>MTPESVMMMGTEAMKVALALAAPLLLVALITGLIISILQAATQINEMTLSFIPKIVAVFIAIIVAGPWMLNLLLDYVRTLFSNLPYIIG[4x];> MIQVTSEQWLYWLHLYFWPLLRVLALISTAPILSERAIPKRVKLGLGIMITLVIAPSLPANDTPLFSIAALWLAMQQILIGIALGFTMQFAFAAVRTAGEFIGLQMGLSFATFVDPGSHLNMPVLARIMDMLAMLLFLTFNGHLWLISLLVDTFHTLPIGSNPVNSNAFMALARAGGLIFLNGLMLALPVITLLLTLNLALGLLNRMAPQLSIFVIGFPLTLTVGIMLMAALMPLIAPFCEHLFSEIFNLLADIVSEMPINNNP;>[5x]MRRLLFLSLAGLWLFSPAAAAQLPGLISQPLAGGGQSWSLSVQTLVFITSLTFLPAILLMMTSFTRIIIVFGLLRNALGTPSAPPNQVLLGLALFLTFFIMSPVIDKIYVDAYQPFSEQKISMQEALDKGAQPLRAFMLRQTREADLALFARLANSGPLQGPEAVPMRILLPAYVTSELKTAFQIGFTIFIPFLIIDLVIASVLMALGMMMVPPATIALPFKLMLFVLVDGWQLLMGSLAQSFYS;>MAAIQGIEGVISQLQATAMAARGQDTHSQSTVSFAGQLHAALDRISDRQAAARVQAEKFTLGEPGIALNDVMADMQKASVSMQMGIQVRNKLVAAYQEVMSMQV[6x];>[5x]MLDRLDAALRFQQEALNLRAQRQEILAANIANADTPGYQARDIDFASELKKVMVRGREETGGVALTLTSSHHIPAQAVSSPAVDLLYRVPDQPSLDGNTVDMDRERTQFADNSLKYQMGLTVLGSQLKGMMNVLQGGN;>MALLNIFDIAGSALAAQSKRLNVAASNLANADSVTGPDGQPYRAKQVVFQVDAAPGQATGGVKVASVIESQAPEKLVYEPGNPLADANGYVKMPNVDVVGEMVNTMSASRSYQANIEVLNTVKSMMLKTLTLGQ[6x];>[11x]MSATASTATQPKPLEWLNRLRANPRIPLIVAGSAAVAIVVAMVLWAKTPDYRTLFSNLSDQDGGAIVAQLTQMNIPYRFANGSGAIEVPADKVHELRLRLAQQGLPKGGAVGFELLDQEKFGISQFSEQVNYQRALEGELARTIETLGPVKSARVHLAMPKPSLFVREQKSPSASVTVTLEPGRALDEGQISAVVHLVSSAVAGLPPGNVTLVDQSGHLLTQSNTSGRDLNDAQLKFANDVESRIQRRIEAILSPIVGNGNVHAQVTAQLDFANKEQTEEHYSPNGDASKATLRSRQLNISEQVGAGYPGGVPGALSNQPAPPNEAPIATPPTNQQNAQNTPQTSTSTNSNSAGPRSTQRNETSNYEVDRTIRHTKMNVGDIERLSVAVVVNYKTLADGKPLPLTADQMKQIEDLTREAMGFSDKRGDTLNVVNSPFSAVDNTGGELPFWQQQSFIDQLLAAGRWLLVLVVAWILWRKAVRPQLTRRVEEAKAAQEQAQVRQETEEAVEVRLSKDEQLQQRRANQRLGAEVMSQRIREMSDNDPRVVALVIRQWMSNDHE;>MDHAIYTAMGAASQTLNQQAVTASNLANASTPGFRAQLNALRAVPVDGLSLATRTLVTASTPGADMTPGQLDYTSRPLDVALQQDGWLVVQAADGAEGYTRNGNIQVGPTGQLTIQGHPVIGEGGPITVPEGSEITIAADGTISALNPGDPPNTVAPVGRLKLVKAEGNEVQRSDDGLFRLTAEAQAERGAVLAADPSIRIMSGVLEGSNVKPVEAMTDMIANARRFEMQMKVITSVDENEGRANQLLSMS[5x]

The bacterial flagellar motor is a huge bidirectional rotary nanomachine that drives rotation of the flagellum for bacterial motility. The cytoplasmic C ring of the flagellar motor functions as the switch complex for the rotational direction switching from counterclockwise to clockwise. The basal body is made up of the LP ring, MS ring, C ring, rod and export apparatus. Here, we present two high-resolution cryo-electron microscopy structures of the C ring-containing flagellar basal body–hook complex from Salmonella Typhimurium, which are in the default counterclockwise state and in a constitutively active CheY mutant-induced clockwise state, respectively.

Given the high fragility of the C ring, we examined several reagents as the media of density gradient centrifugation in the purification of the intact C ring-containing basal body–hook complex in the default CCW state from our previously constructed ΔfliCD strain of S. Typhimurium, which lacks the flagellar filament, thus avoiding effects of the filaments on purification of the motor. Local refinements of the LP ring, MS ring, rod, hook and export apparatus generated their high-quality cryo-EM density maps at the resolutions ranging from 3.0 Å to 4.3 Å. The MS ring is located on the inner membrane, houses the export apparatus and forms the assembly base for the C ring. In the intact C ring-containing basal body–hook complexes, there is one more peptide loop L3, which consists of the residues G310–P322 of FliF and is also extended from the β-collar region of the MS ring, bound in a hydrophobic groove that is formed by the α2–α3 linking loop of FliE6 with the D0 and DC domains of FlgC1 and FlgC6 on the surface of the rod. Thus, there are totally 11 FliF loops that extend from the MS ring to bind the rod in the basal body for torque transmission.>MSQKEVYDAAGFGNPVSRGVHPAIIVVDFSYGFTDLQYPTASDASLQMSRTKEICDLARALEFPVIFTTIAYHPGEIPMLPWLEKSSGMAALLYGSRLVEIDMATGIQPNDVVVVKKGASSFFGSTLSSLLAGTNTDTVVVTGATTSGCVRATVVDAVQSGFKVLVPADCCADRAKG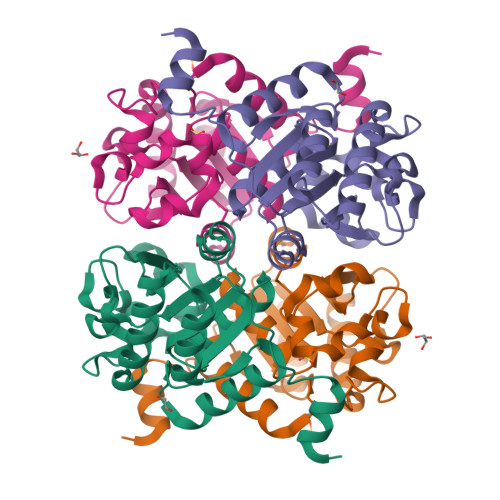PHEASLYDIQQKYGDVTDSDDILKWLRSVAG[2x]>[2x]MGPGTWENMAFAQDSSAINNIDGYLSYTDWYRPYGTSQDGKTWYKTTAMDWRPLLMYIWPSKDVQAQFIKYFVNNGYENANYGLTKDTVANINKDTNTTVLANMAQNLRYVIEQSIAANKGTSKLANDINSFAATVPELSASSELSLQSMPNYRPDKSGTIDSDQVIFVNNNSKDPRKGNTSYADSNYRLMNRTINNQAGNNNSDNSPELLVGNDIDNSNPVVQAENLNWEYFLLNYGKLMGYNPDGNFDG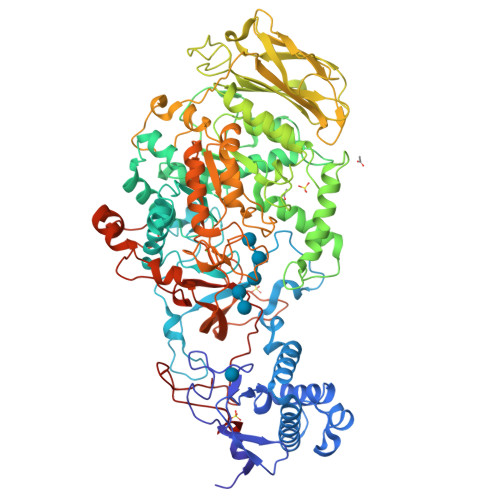FRVDAADNIDADVLDQMGQLMNDMYHTKGNPQNANDHLSYNEGYHSGAAQMLNEKGNPQLYMDSGEFYTLENVLGRANNRDNIGNLITNSIVNRQNDTTENEATPNWSFVTNHDQRKNLINRLIIKDHSNIPDIMGSAYKVEYANQAWQEFYADQEKTNKQYAQYNVPAQYAILLSNKDTVPQVYYGDLYNETAQYMQEKSIYYDAITTLMRARKQFVSGGQTMTKLNNNLLASVRYGKGVVDANSNGTDKLSRTSGMAVLVGNDSNMAQQSVAINMGRAHANQQYRNLIDTTENGLTYDADNSENPAILTTDSNGILKVTVKGYSNPYVSGYLGVWVPVISGDQDVTTNASDVVANKEKTFESNAALDSHMIYEDFSLFQPEPTSVENHAYNVIAKNASLFSDLGITDFWMAPAYTPFGRSRYNEGYSMTDRYNLGTTANPTKYGSGEELANTIAALHKAGLKVQEDIVMNQMIGFSGQEAVTVTRTNNRGMQIHVNGQTYANQIYFAYTTGGGNGQETYGGKYLAELQKNYPDLFTTKAISTGVAPDPTVRINKWSAKYQNGTSLQNIGIGLAVKLANGDYAYLNSGDNKAFNTLLPTAIS>MRDWVIPPISCPENEKGEFPKNLVQIKSNRDKETKVFYSITGQGADKPPVGVFIIERETGWLKVTQPLDREAIAKYILYSHAVSSNGEAVEDPMEIVITVTDQNDNRPEFTQEVFEGSVAEGAVPGTSVMKVSATDADDDVNTYNAAIAYTIVSQDPELPHKNMFTVNRDTGVISVLTSGLDRESYPTYTLVVQ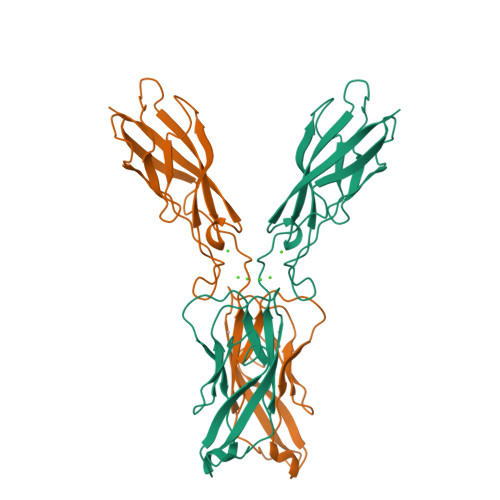AADLQGEGLSTTAKAVITVKDINDNAPVFNPS[2x]>MRNRREVSKLLSERVLLLDGAYGTEFMKYGYDDLPEELNIKAPDVVLKVHRSYIESGSDVILTNTFGATRMKLRKHGLEDKLDPIVRNAVRIARRAAGEKLVFGDIGPTGELPYPLGSTLFEEFYENFRETVEIMVEEGVDGIIFETFSDILELKAAVLAAREVSRDVFLIAHMTFDEKGRSLTGTDPANFAITFDELDIDALGINCSLGPEEILPIFQELSQYTDKFLVVEPNAGKPIVENGKTVYPLKPHDFAVHIDSYYELGVNIFGGCCGTTPEHVKLFRKVLGNRKPLQRKKKRIFAVSSPSKLVTFDHFVVIGERINPAGRKKLWAEMQKGNEEIVIKEAKTQVEKGAEVLDVNFGIESQIDVRYVEKIVQTLPYVSNVPLSLDIQNVDLTERALRAYPGRSLFNSAKVDEEELEMKINLLKKYGGTLIVLLMGKDVPKSFEERKEYFEKALKILERHDFSDRVIFDPGVLPLGAEGKPVEVLKTIEFISSKGFNTTVGLSNLSFGLPDRSYYNTAFLVLGISKGLSSAIMNPLDETLMKTLNATLVILEKKELPR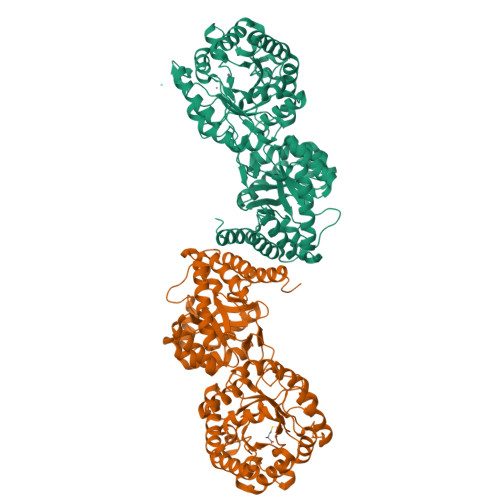AEVK[2x]> TG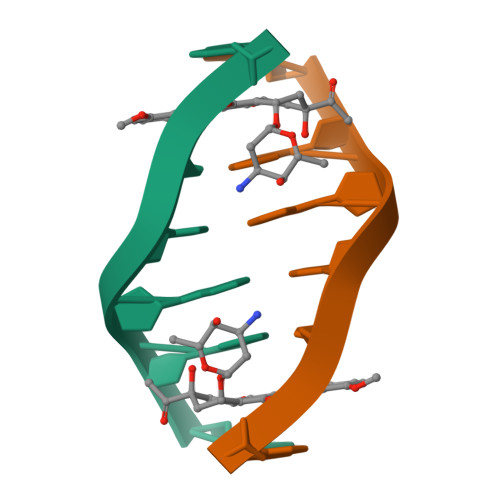ATCA>MSLSAPRITRVETAAIRAVGPSVLVRVWAGDEHGLGECYPSAPAAGIHHIVMNMEEQLLGEDPRDVERLYEKMRRWNIFTGGQAGAVITALSGIETALWDLAGKLQGVPVYRLLGGAFRRRVRLYADCNAGTVDAAAHHIEGGLFEEGSNEEYIAVAREAVERGFDAIKLDVDDITGPLHRDFWNGAISPREHEAMVARVAAVREAVGPEVEVAIDMHGRFDIPSSIRFARAMEPFGLLWLEEPTPPENLDALAEVRR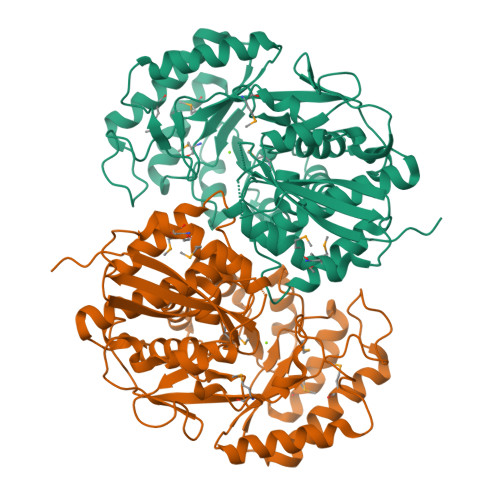STSTPICAGENVYTRFDFRELFAKRAVDYVMPDVAKCGGLAEAKRIANLAELDYIPFAPHNVSSPVGTVAAAHVCAAVSNFAVLEWHAIDMPHWEDFVRYPGGPVIREGHIELTEEPGLGLELDEEAAFEHRHEKGGVPFFGRTEGHHHHHH[2x]In vertebrates, a group of at least 16 inner kinetochore proteins, collectively identified as constitutive centromere-associated network (CCAN), neighbors the CENP-A nucleosome. The CCAN (whose subunits are indicated as ‘CENP’—for centromeric protein—followed by a letter) interacts with the outer kinetochore and contributes to maintain centromere identity by participating in CENP-A loading at every new cell division cycle. In this study, we concentrate on four additional CCAN subunits, CENP-H, CENP-I, CENP-K, and CENP-M. These proteins have been shown to be proximal to the subunits of the CENP-T/W/X/S, CENP-O/P/Q/U, and CENP-N/L complexes in cell lysates, but their organization and pattern of interactions remain unclear. In this study, we elucidate the molecular basis of CENP-M's essential function in kinetochore assembly.

We generated crystals of residues 1–171 of CENP-M (a fragment identified by limited proteolysis) and determined their crystal structure by the SAD (single-wavelength anomalous diffraction) method to a resolution of 1.5 Å using a SeMet derivative. The structure of CENP-M1–171 is globular and consists of a five-stranded parallel β-sheet surrounded by six α-helices. Structural superposition with representative members of different families identified Rab proteins as the closest structural homologs of CENP-M. Thus, HsCENP-M has the fold of a small GTPase, but may be unable to bind (and therefore hydrolyze) GTP. Experiments with MANT nucleotides confirmed this prediction directly. CENP-M is devoid of all essential sequence signatures associated with nucleotide binding, hydrolysis and conformational switching of small GTPases. An invariant feature of CENP-M is the presence of leucine at position 52 (of HsCENP-M), equivalent to Gln61 (Q61) at the end of the Switch II region of Ras. Thus, the first step leading CENP-M to diverge from genuine GTPases might have been an impairment of GTP hydrolysis, followed by the loss of other features associated with GTP handling. In conclusion, we identify CENP-M as a ‘pseudo G-protein’, in analogy to inactive kinase domains, indicated with the term ‘pseudokinase’. CENP-M (∼20 kDa) elutes as expected for a monomeric species.

>[2x]GPLGSMSVLRPLDKLPGLNTATILLVGTEDALLQQLADSMLKEDCASELKVHLAKSLPLPSSVNRPRIDLIVFVVNLHSKYSLQNTEESLRHVDASFFLGKVCFLATGAGRESHCSIHRHTVVKLAHTYQSPLLYCDLEVEGFRATMAQRLVRVLQICAGHVPGVSALNLLSLLRS(1R,2S)-2-(5-thioxo-4,5-dihydro-1H-1,2,4-triazol-3-yl)cyclohexanecarboxylic acid | C9 H13 N3 O2 S | 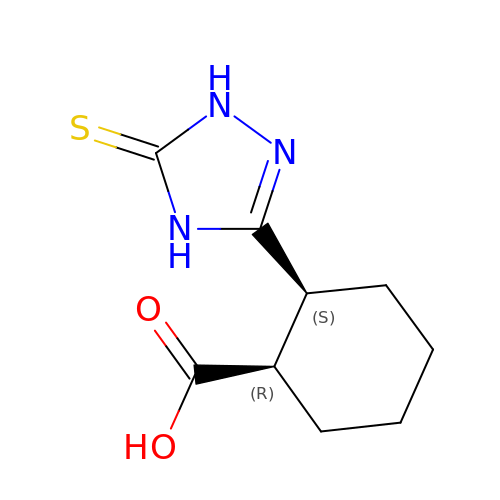DYLXWYPNDHPRPQ-NTSWFWBYSA-N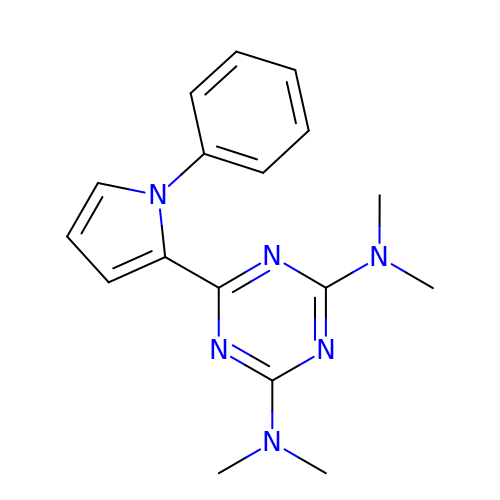~{N}2,~{N}2,~{N}4,~{N}4-tetramethyl-6-(1-phenylpyrrol-2-yl)-1,3,5-triazine-2,4-diamine | C17 H20 N6 | YGYIXUFMSVWSAM-UHFFFAOYSA-N> MKRDKTSDLVEEYFEAHSSSKVLTSDRTLQKLKRAKLDQQTLRNLLSKVSPSFSAELKQLNQQYEKLFHKWMLQLHLGFNIVLYGLGSKRDLLERFRTTMLQDSIHVVINGFFPGISVKSVLNSITEEVLDHMGTFRSILDQLDWIVNKFKEDSSLELFLLIHNLDSQMLRGEKSQQIIGQLSSLHNIYLIASIDHLNAPLMWDHAKQSLFNWLWYETTTYSPYTEE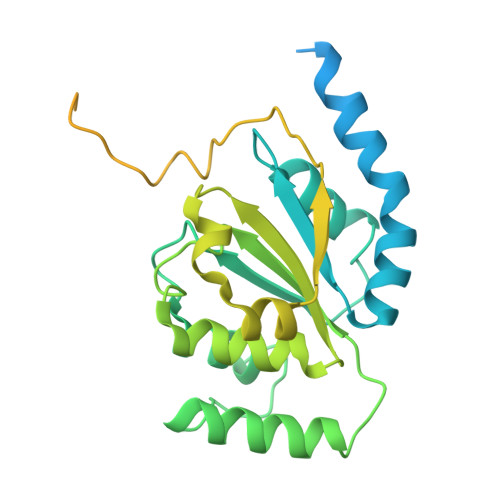TSYENSLLVKQSGSLPLSSLTHVLRSLTPNARGIFRLLIKYQLDNQDNPSYIGLSFQDFYQQCREAFLVNSDLTLRAQLTEFRDHKLIRTKKGTDGVEYLLIPVDNGTLTDFLEKEEEEA~{N},1-dimethyl-5-[[4-[3-methyl-4-[[(3~{R})-piperidin-3-yl]amino]pyrazol-1-yl]pyrimidin-2-yl]amino]indazole-3-carboxamide 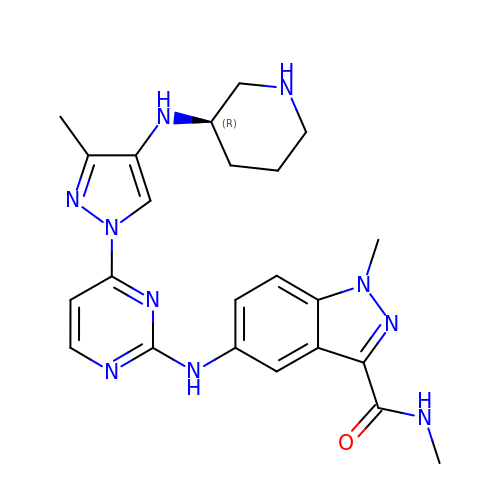| C23 H28 N10 O | CGMCYALTKDQISD-MRXNPFEDSA-N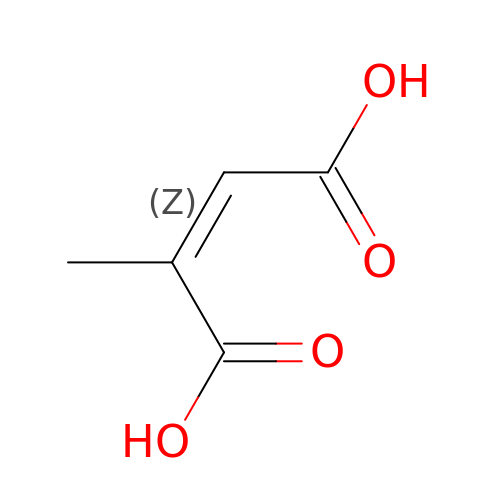(~{Z})-2-methylbut-2-enedioic acid | C5 H6 O4 | HNEGQIOMVPPMNR-IHWYPQMZSA-N>[4x]GMTTKD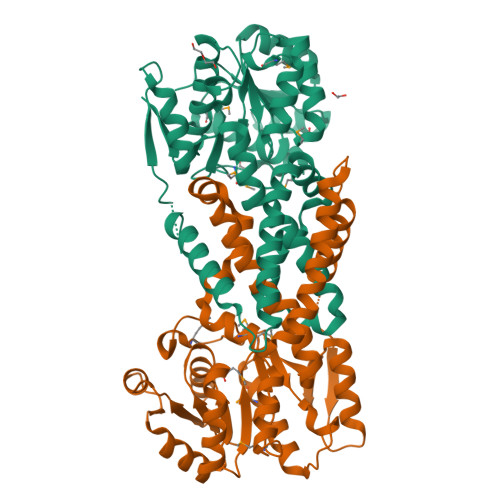ISRPVCILGLGLIGGSLLRDLHAANHSVFGYNRSRSGAKSAVDEGFDVSADLEATLQRAAAEDALIVLAVPMTAIDSLLDAVHTHAPNNGFTDVVSVKTAVYDAVKARNMQHRYVGSHPMAGTANSGWSASMDGLFKRAVWVVTFDQLFDGTDINSTWISIWKDVVQMALAVGAEVVPSRVGPHDAAAARVSHLTHILAETLAIVGDNGGALSLSLAAGSYRDSTRVAGTDPGLVRAMCESNAGPLVKALDEALAILHEAREGLTAEQPNIEQLADNGYRSRIRYEARSGQRRAKESVSPTITSSRPVLRLHPGTPNWEKQLIHAETLGARIEVF>GMELRVGNRYRLGR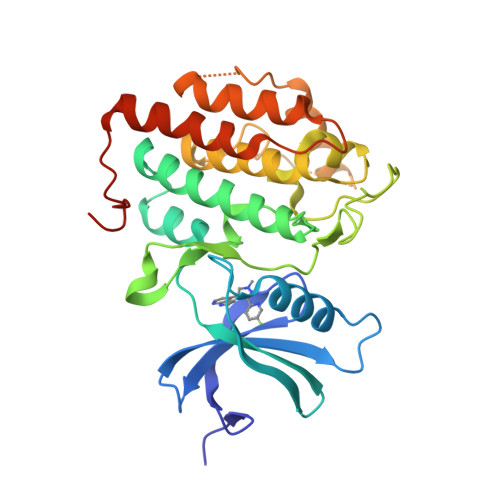KIGSGSFGDIYLGTDIAAGEEVAIKLECVKTKHPQLHIESKIYKMMQGGVGIPTIRWCGAEGDYNVMVMELLGPSLEDLFNFCSRKFSLKTVLLLADQMISRIEYIHSKNFIHRDVKPDNFLMGLGKKGNLVYIIDFGLAKKYRDARTHQHIPYRENKNLTGTARYASINTHLGIEQSRRDDLESLGYVLMYFNLGSLPWQGLKAATKRQKYERISEKKMSTPIEVLCKGYPSEFATYLNFCRSLRFDDKPDYSYLRQLFRNLFHRQGFSYDYVFDWNMLKFGASR[2x]>[4x]ETELAFLYERDIYRLLAECDNSRNPDLGLIVRICLATGARWSEAETLTQSQVMPYKITFTNTKSKKNR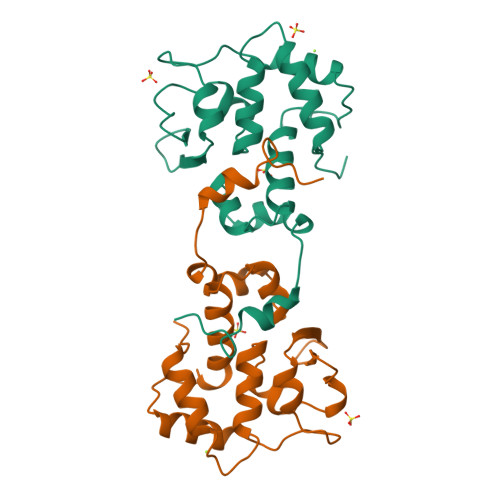TVPISDELFDMLPKKRGRLFNDAYESFENAVLRAEIELPKGQLTHVLRHTFASHFMMNGGNILVLKEILGHSTIEMTMRYAHFAPSHLESAVKFNPLSNPAQ>[4x]MDQKPQPAKTHATEVTVLEGKTMGTFWRASIPGIDAKRSAELKEKIQTQLDADDQLLSTYKKDSALMRFNDSQSLSPWPVSEAMADIVTTSLRIGAKTDGAMDITVGPLVNLWGFGPEQQPVQIPSQEQIDAMKAKTGLQHLTVINQSHQQYLQKDLPDLYVDLSTVGKGYAADHLARLMEQEGISRYLVSVGGALNSRGMNGEGLPWRVAIQKPTDKENAVQAVVDINGHGISTSGSYRNYYELDGKRLSHVIDPQTGRPIEHNLVSVTVIAPTALEADAWDTGLMVLGPEKAKEVVRREGLAVYMITKEGDSFKTWMSPQFKSFLVSEKNLEHHHHHH

We recently reported a flavin‐trafficking protein (Ftp) in the syphilis spirochete Treponema pallidum (Ftp_Tp) as the first bacterial metal‐dependent FAD pyrophosphatase that hydrolyzes FAD into AMP and FMN in the periplasm. Orthologs of Ftp_Tp in other bacteria (formerly ApbE) appear to lack this hydrolytic activity; rather, they flavinylate the redox subunit, NqrC, via their metal‐dependent FMN transferase activity. In the current study, we identified a bimetal center in the crystal structure of Escherichia coli Ftp (Ftp_Ec) and show via mutagenesis that a single amino acid substitution converts it from an FAD‐binding protein to a Mg2+‐dependent FAD pyrophosphatase (Ftp_Tp‐like). A high‐resolution structure of the Ftp‐mediated flavinylated protein of Shewanella oneidensis NqrC identified an essential lysine in phosphoester‐threonyl‐FMN bond formation in the posttranslationally modified flavoproteins.

We were also unsuccessful in our attempt to obtain an FAD‐bound structure of the Ftp_EcE169K protein variant (this residue is analogous to the active‐site residue K165 in Ftp_Tp), but once again obtained a structure that was determined at a higher resolution than wild‐type (1.75 vs. 1.88 Å) with a similarly improved final Rfree parameter. There are four monomers in the asymmetric unit of each crystal structure, and the r.m.s.d. of the monomers within each structure ranges from 0.5 to 1.6 Å and 0.3 to 1.6 Å, respectively, between the two structures for approximately 300 Cα carbons. John Wiley & Sons, LtdIn the site previously denoted in the Ftp_Tp structure as metal binding site 1, a single metal ion is bound in the wild‐type and Ftp_EcE169K protein variant structures. Aided by the high resolution of our structural data, two water molecules were observed bound to each metal ion and thus the coordination number for the metal is seven, consistent with a Ca2+ rather than a Mg2+ ion as observed in the Ftp_Tp structures. Refinement of the metal in this site as a Mg2+ ion resulted in large positive peaks in a difference electron‐density map; these peaks disappeared when modeled as a Ca2+ ion. Thus, in agreement with the original structure determination, we have assigned these as Ca2+ ions. Superposition of three representative Ftp_Ec monomers illustrates the inherent flexibility of the loop region near the active site comprising residues 237–253.> HMLEAKFEEASLFKRIIDGFKDCVQLVNFQCKEDGIIAQAVDDSRVLLVSLEIGVEAFQEYRCDHPVTLGMDLTSLSKILRCGNNTDTLTLIADNTPDSIILLFEDTKKDRIAEYSLKLMDIDADFLKIEELQYDSTLSLPSSEFSKIVRDLSQLSDSINIMITKETIKFVADGDIGSGTVIIKPFVDMEHPETSIKLEMDQPVDLTFGAKYLLDIIKGSSLSDRVGIRLSSEAPALFQFDLKSGFLQFFLAPKFNDEE

Proliferating cell nuclear antigen (PCNA) is a protein that is essential for many DNA metabolic processes including DNA replication, base excision repair, nucleotide excision repair, mismatch repair, and recombination. PCNA is a ring-shaped homo-trimer that acts as a sliding clamp that encircles DNA forming a scaffold for binding numerous proteins involved in DNA metabolism. PCNA is required for translesion synthesis (TLS), which is a pathway for bypassing DNA damage during replication. The subunit interface of PCNA is comprised of two anti-parallel β strands: strand I1 (residues 109 to 117) in domain 1 of one subunit and strand D2 (residues 175 to 183) in domain 2 of the adjacent subunit.

To better understand the role of the subunit interface in translesion synthesis and in other DNA metabolic processes, we used random mutagenesis to generate a series of PCNA mutant proteins with substitutions in either of these two β strands. We first measured the growth rate of these 17 strains in liquid media. Twelve of these strains (A112G, Y114F, S115E, S115G, S115V, S177G, S177L, S177V, G178L, G178M, S178T, and V180A) had slower growth rates than the wild type strain of approximately 4 to 5 hours. The remaining five strains had growth rates similar to the wild type strain of approximately 2 to 3 hours. We next measured the UV sensitivity of these 17 strains. All 17 strains had increased sensitivities to UV radiation to some extent compared to the wild type except G178M. We then examined the rates of spontaneous mutagenesis and the rates of UV-induced mutagenesis of these 17 strains as well as E113G and G178S. By contrast, all 17 strains, except the S177G, S179A, and V180A mutant strains, had statistically significant defects in the rate of UV-induced mutagenesis (with p values less than 0.05). Five of these strains (S115N, S177V, S179R, S179T, and I181R) had complete defects in UV-induced mutagenesis similar to that observed with the K164R control strain. A defect in UV-induced mutagenesis is a characteristic indicator of a defect in error-prone TLS.>[6x]MQK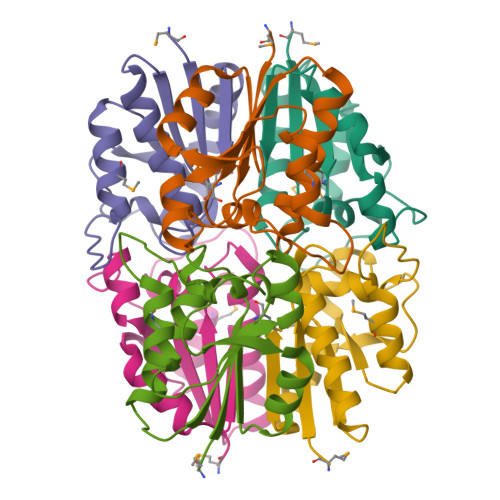IVIVANGAPYGSESLFNSLRLAIALREQESNLDLRLFLMSDAVTAGLRGQKPGEGYNIQQMLEILTAQNVPVKLCKTCTDGRGISTLPLIDGVEIGTLVELAQWTLSADKVLTF Iodomethane | C H3 I | 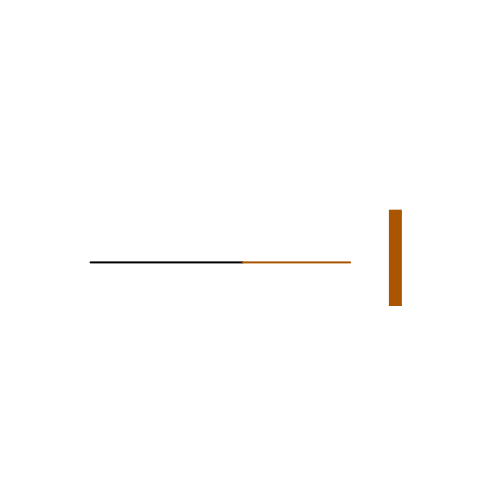INQOMBQAUSQDDS-UHFFFAOYSA-N> MQINQVRPKLPLLKILHAAGAQGEMFTVKEVMHYLGQYIMVKQLYDQQEQHMVYCGGDLLGELL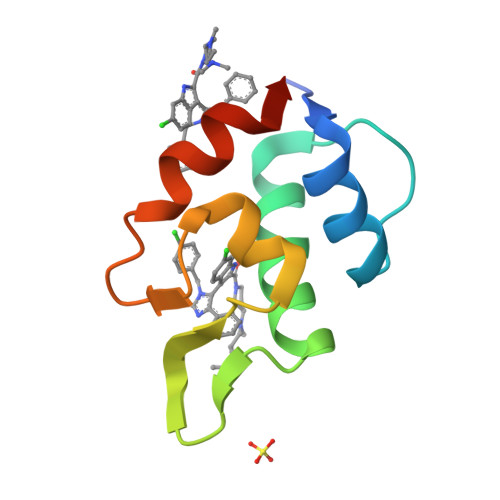GRQSFSVKDPSPLYDMLRKNLVTLAT> HGFVDNATIGGQFYQFYQPYQDPFMGSPPDRISRKIPGNGPVEDVTSLAIQCNADSAPAKLHASAAAGSTVTLRWTIWPDSHVGPVITYMARCPDTGCQDWTPSASDKVWFKIKEGGREGTSNVWAATPLMTA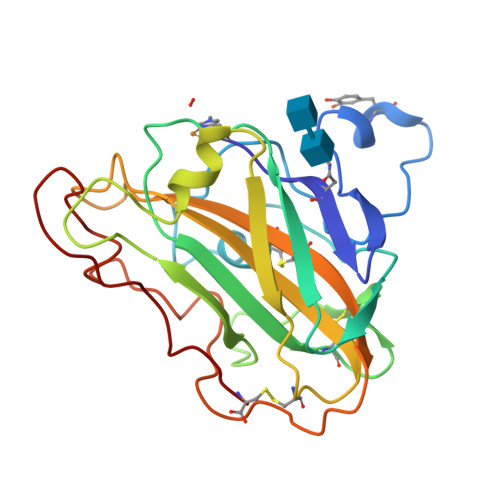PANYEYAIPSCLKPGYYLVRHEIIALHSAYSYPGAQFYPGCHQLQVTGSGTKTPSSGLVSFPGAYKSTDPGVTYDAYQAATYTIPGPAVFTC;> HGFVDNATIGGQFYQFYQPYQDPYMGSPPDRISRKIPGNGPVEDVTSLAIQCNADSAPAKLHASAAAGSTVTLRWTIWPDSHVGPVITYMARCPDTGCQDWTPSASDKVWFKIKEGGREGTSNVWAATPLMTAPANYEYAIPSCLKPGYYLVRHEIIALHSAYSYPGAQFYPGCHQLQVTGSGTKTPSSGLVSFPGAYKSTDPGVTYDAYQAATYTIPGPAVFTC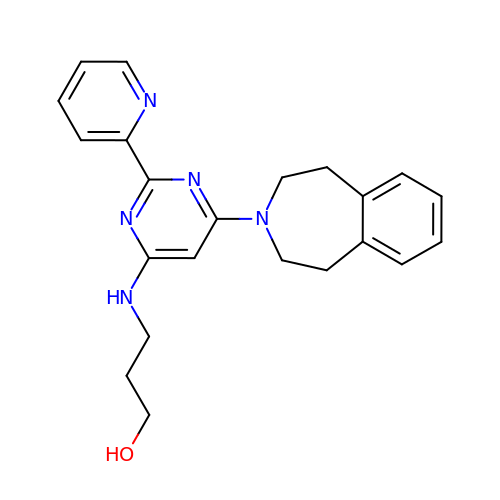3-[[2-pyridin-2-yl-6-(1,2,4,5-tetrahydro-3-benzazepin-3-yl)pyrimidin-4-yl]amino]propan-1-ol | C22 H25 N5 O | XLIJLZCIQJERJQ-UHFFFAOYSA-N>MNSE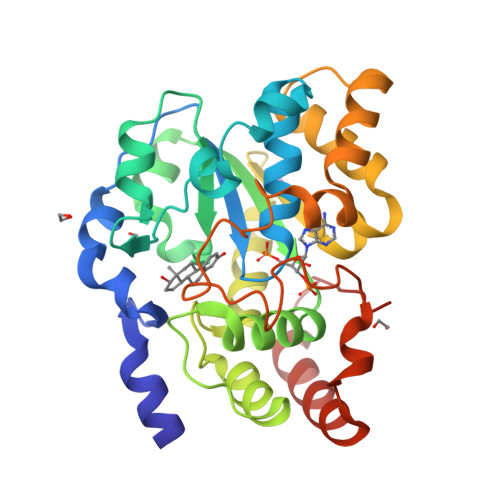LDYYEKFEEVHGILMYKDFVKYWDNVEAFQARPDDLVIATYPKSGTTWVSEIVYMIYKEGDVEKCKEDVIFNRIPFLECRKENLMNGVKQLDEMNSPRIVKTHLPPELLPASFWEKDCKIIYLCRNAKDVAVSFYYFFLMVAGHPNPGSFPEFVEKFMQGQVPYGSWYKHVKSWWEKGKSPRVLFLFYEDLKEDIRKEVIKLIHFLERKPSEELVDRIIHHTSFQEMKNNPSTNYTTLPDEIMNQKLSPFMRKGITGDWKNHFTEALNEKFDKHYEQQMKESTLKFRTEI[2x]> GSHMDNQCTVQVRLELGHRAQLRKKPTTEGFTHDWMVFVRGPEQCDIQHFVEKVVFWLHDSFPKPRRVCKEPPYKVEESGYAGFIMPIEVHFKNKEEPRKVCFTYDLFLNLEGNPPVNHLNHLRCEKL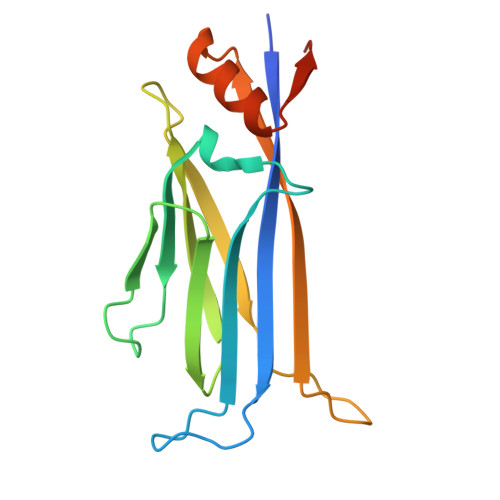TFNNPTTEFRYKLLRAGGVMVMPEGAHHHHHH>GSHMAAGGDHGSPDSYRSPLASRYASPEMCFVFSDRYKFRTWRQLWLWLAEAEQTLGLPITDEQIQEMKSNLENIDFKMAAEEEKRLRHDVMAHVHTFGHCCPKAAGIIHLGATSCYVGDNTDLIILRNALDLLLPKLARVISRLADFAKERASLPTLGFTHFQPAQLTTVGKRCCLWIQDLCMDLQNLKRVRDDLRFRGVKGTTGTQASFLQLFEGDDHKVEQLDKMVTEKAGFKRAFIITGQTYTRKVDIEVLSVLASLGASVHKICTDIRLLANLKEMEEPFEKQQIGSSAMPYKRNPMRSERCCSLARHLMTLVMDPLQTASVQWFERTLDDSANRRICLAEAF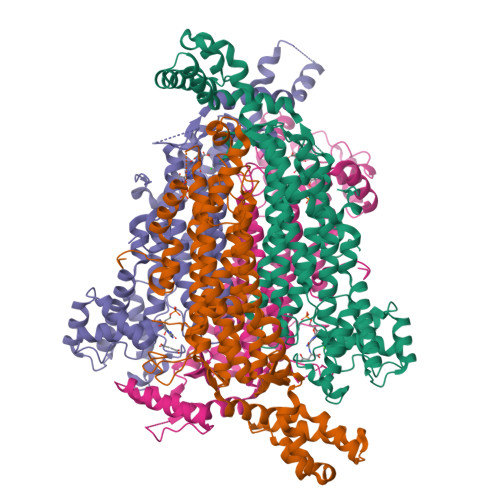LTADTILNTLQNISEGLVVYPKVIERRIRQELPFMATENIIMAMVKAGGSRQDCHEKIRVLSQQAASVVKQEGGDNDLIERIQADAYFSPIHSQLDHLLDPSSFTGRASQQVQRFLEEEVYPLLKPYESVMKVKAELCL[8x]>MSTSSSSQSLKIGIVGFGNFGQFLAKTMIKQGHTLTATSRSDYSELCLQMGIHFFRDVSAFLTADIDVIVLCTSILSLSEVVGSMPLTSLKRPTLFVDVLSVKEHPRELLLRELPEDSDILCTHPMFGPQTAKNGWTDHTFMYDKVRIRDEVICSNFIQIFATEGCKMVQMSC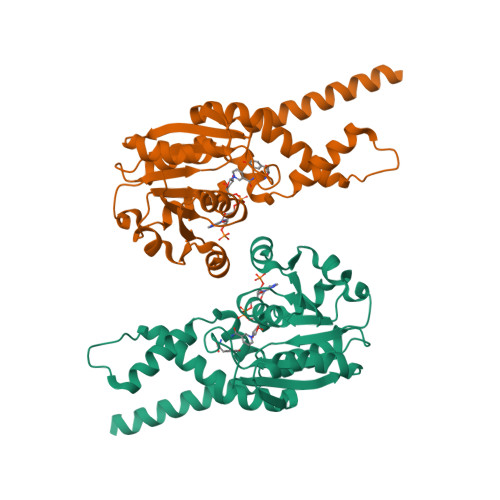EEHDRAAAKSQFITHTIGRTLGEMDIQSTPIDTKGFETLVKLKETMMRDSFDLYSGLFVYNRFARQELENLEHALHKVKETLMIQRTNGEQGHKRTES[2x]> GGACAUA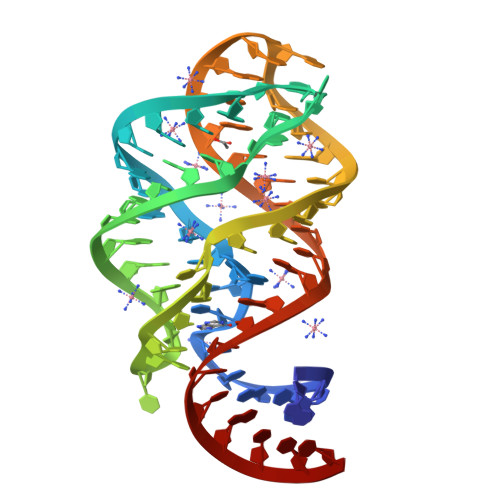CAAUCGCGUGGAUAUGGCACGCAAGUUUCUGCCGGGCACCGUAAAUGUCCGACUAUGUCC2-deoxy-2,2-difluoro-beta-D-lyxo-hexopyranose | 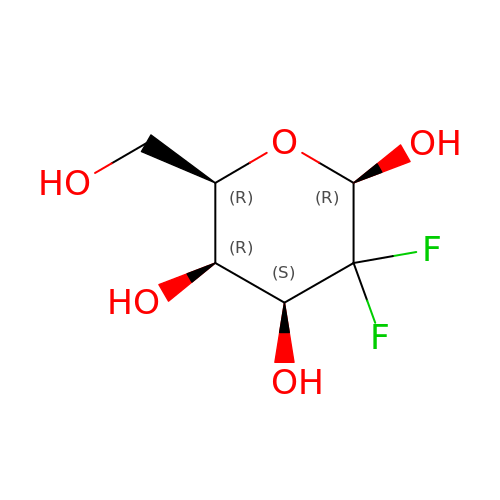C6 H10 F2 O5 | SHBCJQOMZTUYEL-MGCNEYSASA-N>[2x]MRTLLDLDPKGKRVLVRVDYNVPVQDGKVQDETRILESLPTLRHLLAGGASLVLLSHLGRPKGPDPKYSLAPVGEALRAHLPEARFAPFPPGSEEARREAEALRPGEVLLLENVRFEPGEEKNDPELSARYARLGEAFVLDAFGSAHRAHASVVGVARLLPAYAGFLMEKEVRALSRLLKDPERPYAVVLGGAKVSDKIGVIESLLPRIDRLLIGGAMAFTFLKALGGEVGRSLVEEDRLDLAKDLLGR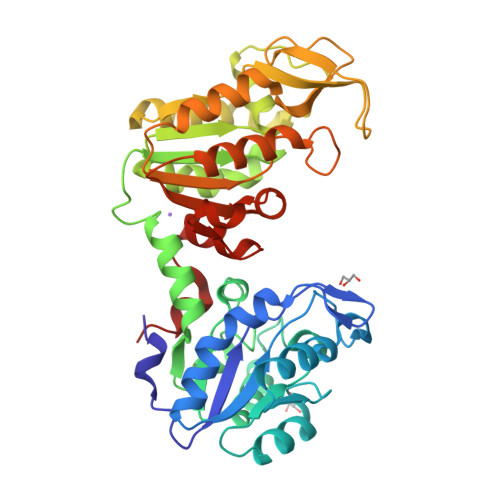AEALGVRVYLPEDVVAAERIEAGVETRVFPARAIPVPYMGLDIGPKTREAFARALEGARTVFWNGPMGVFEVPPFDEGTLAVGQAIAALEGAFTVVGGGDSVAAVNRLGLKERFGHVSTGGGASLEFLEKGTLPGLEVLEG> SSSNYCNQMMKSRNLTKDRCKPVNTFVHESLADVQAVCSQKNVACKNGQTNCYQS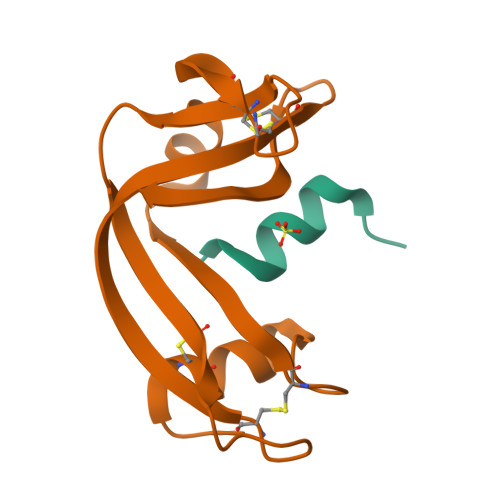YSTMSITDCRETGSSKYPNCAYKTTQANKHIIVACEGNPYVPVHFDASV;> KETAAAKFERQHFDSX>SMNYFVGNSLGVNLTGIEKAIINRLNLFKEMGRPAQCVFLSWNRYLYRNAQNYITSSDYINMYDFFQEATYLERNEPFDWLSYWTDECHYTLKHVENSHDFRIYDQERFLMYAHFQDPKYRILDYVNHFDSQRRKVKRDFYDVRGFLSCSRILVDKQQTLCEFFYNPEGDTKLEKYFSYKDGKPEVQKIIVYYANKQYFFNNETELGAFFIKQLYQHGDLFFSDRNVYTAPIFNLTPESIPVVAVLHSTHIKNIDALDSSPFKNVYKAMFENLSRYRAIIVSTEQQKLDVEKRINHTIPVVNIPVGYSETIDTPVQTLDQRSVKLISVARYSPEKQLHQQIELIKRLVSYVPKIELHMYGFGSESKKLNELIQKYGLENHVYLRGFLSNLDQEYSDAYLSLITSNMEGFSLALLESLAHGVPVISYD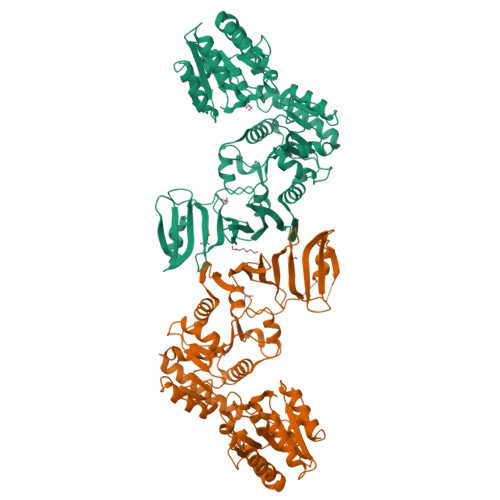IKYGPNELITSDFNGYLITKNDEDALFDKVKYVIDHPEVQQRLSKGSLAKAQQYSKASLIKQWDQFVRLILEHHHHHH[2x]>MHELTIYHFMSDKLNLYSDIGNIIALRQRAKKRNIKVNVVEINETEGITFDECDIFFIGGGSDREQALATKELSKIKTPLKEAIEDGMPGLTICGGYQFLGKKYITPDGTELEGLGILDFYTESKTNRLTGDIVIESDTFGTIVGFENHGGRTYHDFGTLGHVTFGYGNNDEDKKEGIHYKNLLGTYLHGPILPKNYEITDYLLEKACERKGIPFEPKEIDNEAEIQAKQVLIDRANRQKKSR[2x]

Recently, MurT and GatD enzymes were identified as responsible for catalyzing glutamate amidation in S. aureus PG stem peptides. Moreover, in vitro experiments showed that the MurT-GatD complex catalyzes glutamate amidation of lipid II using L-glutamine as a direct amine donor, when ATP and Mg2+ were present. GatD shows high sequence homology to the glutaminase domain of glutamine amidotransferase (GATase) enzymes, in particular to cobyric acid synthase, which is involved in cobalamin biosynthesis.

The crystal structure was solved at 1.85 Å resolution, unraveling singular features of GATase architecture and important residues at the active site. GatD crystallized in P212121 space group, with 2 molecules in the asymmetric unit, forming a non-physiological dimer via non-crystallographic symmetry operations (validated by visual inspection and using PISA software). The S. aureus GatD structure here reported was crystallized without its synthase domain (MurT), consequently, in an unproductive enzymatic form. The S. aureus GatD crystal structure shows the characteristic β-sheet core composed by six strands (β1, β2, β3, β4, β10 and β11), all parallel except for β10. Interestingly, GatD holds an extra 17 residues long α-helix (α7) at the C-terminal that is absent in all GATases characterized so far. An important difference between the S. aureus GatD and other GATases so far characterized, is the absence of the glutamate residue that usually completes the catalytic triad (E174 in S. marcescens AS protein). In the structure here reported, glutamate is replaced by a glycine (G190), thereby eliminating any possible polarization effect upon the catalytic histidine H189. The amino acid molecule is found at the surface of the protein, at 8.6 Å from the nucleophilic thiol group of C94, only interacting with R128 from molecule A. The amide oxygen of the free glutamine is establishing hydrogen bonds with the guanidinium group of R128, with bond distances of 3.3 Å and 2.7 Å. The GatD-glutamine complex here reported shows the Y17 side chain nearly co-planar to the H189 imidazole ring and establishing a hydrophobic interaction with C94. In this conformation, Y17 is obstructing the access of the free glutamine to the active site.>[2x]SQSTRKKSRRNKWHFGVRCRGDAPEILLAVYRALQRAG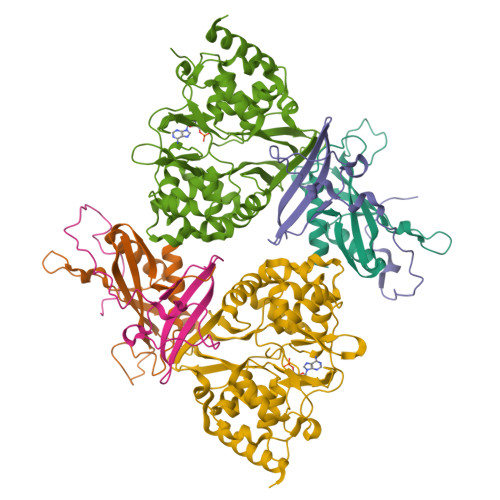AQFTVPKPVNGKYRSDMYTIKSRWEIPHCKREGKNTYAYIELQLYEVMPGCFMLDVKSNGYKDIYSHPERTADHGMDDLKSSFPFLDLCAMLVCKLFSA;>MSESEQYSTEIPAFLTSNTLQELKLPKPPSLPPHLEKCILNSNTAYKEDQSVLPNPNHVLLNHLAAANTQLGVLALSATTRYHRKYVTTAMFKNFDV[2x];>[2x]MDVQETQKGALKEIQAFIRSRTSYDVLPTSFRLIVFDVTLFVKTSLSLLTLNNIVSAPLWDSEANKFAGLLTMADFVNVIKYYYQSSSFPEAIAEIDKFRLLGLREVERKIGAIPPETIYVHPMHSLMDACLAMSKSRARRIPLIDVDGETGSEMIVSVLTQYRILKFISMNCKETAMLRVPLNQMTIGTWSNLATASMETKVYDVIKMLAEKNISAVPIVNSEGTLLNVYESVDVMHLIQDGDYSNLDLSVGEALLKRPANFDGVHTCRATDRLDGIFDAIKHSRVHRLFVVDENLKLEGILSLADILNYIIYDKTTTPGVPEQTDNFESAV>MISNDHLKRLASTSAVMSCTLGKATCLGMDKICSPLADNDVTQRKTQIICTIGPSCNNVESLIGLIDKGMSVARLNFSHGDHESHFKTLQNIREAAKARPHSTVGIMLDTKGPEIRTGMLEGGKPIELKAGQTLKITTDYSMLGNSECISCSYSLLPKSVQIGSTVLIADGSLSTQVLEIGDDFIVCKVLNSVTIGERKNMNLPGCKVHLPIIGDKDRHDIVDFALKYNLDFIALSFVQNGADVQLCRQIIS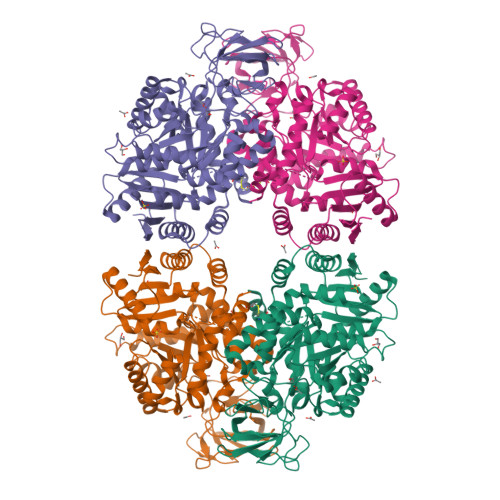ENTQYSNGIPSSIKIISKIENLEGVINFDSICSESDGIMVARGDLGMEIPPEKIFVAQKCMISKCNVAGKPVVTATQMLESMIKSNRPTRAEMTDVANAVLDGSDCVMLSGETANGAFPFDAVNVMSRVCAQAETCIDYPVLYHAIHSSVPKPVAVPEAIACSAVESAHDVNAKLIITITETGNTARLISKYRPSQTIIACTAKPEVARGLKIARGVKTYVLNSIHHSEVVISNALALAKEESLIESGDFAIAVHGVKESCPGSCNLMKIVRCP[2x]> XSLSDKDKAAVRALWSKI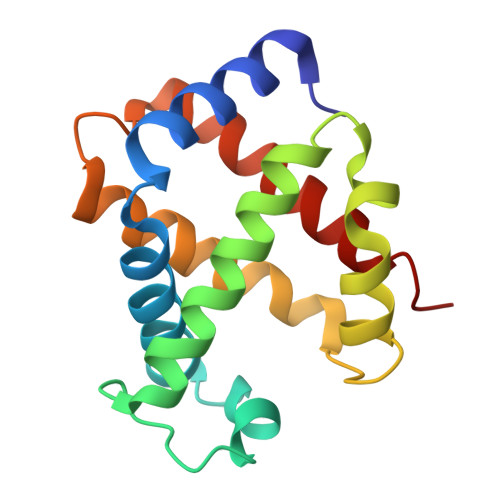GKSADAIGNDALSRMIVVYPQTKTYFSHWPDVTPGSPHIKAHGKKVMGGIALAVSKIDDLKTGLMELSEQHAYKLRVDPANFKILNHCILVVISTMFPKEFTPEAHVSLDKFLSGVALALAERYR>GSISTAVIDAINSGATLKDINAIPDD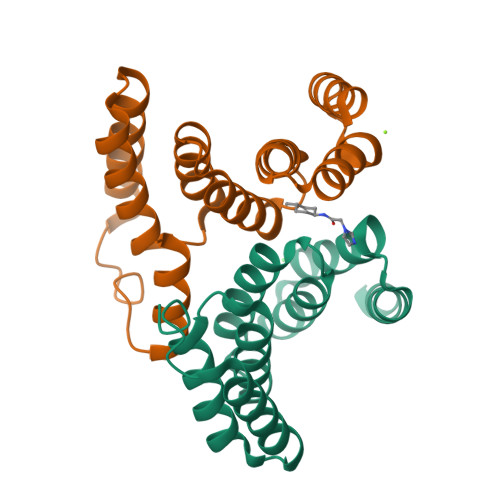MMDDIYSYAYDFYNKGRIEEAEVFFRFLCIYDFYNVDYIMGLAAIYQIKEQFQQAADLYAVAFALGKNDYTPVFHTGQCQLRLKAPLKAKECFELVIQHSNDEKLKIKAQSYLDAIQ[2x]> HMSQAPNDPIEQYEYAQQLLASNKAEASPDTRYWLEQSANQGYL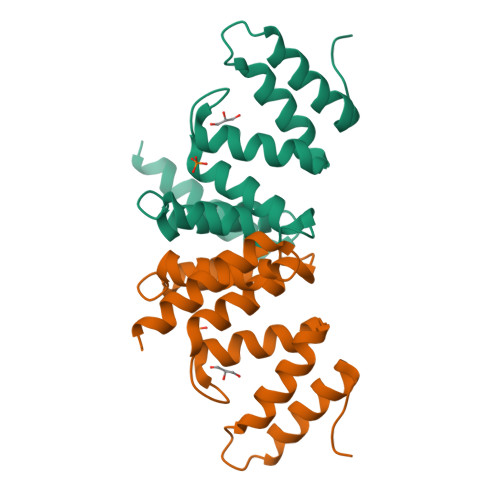PAQKQLANDFAKGINGEKNETQALYWLTSIALNDPTDQGFLLANFIQRNQDKVTTSQLTEALYQMASQHNPAAEQAYNQLLEQRFNQLR> MIRAVFFDSPGTLNSVEGHAKMHLKIMEEVLGDYPLNPKTLLDEYNKLTREAFSNYAGKPYRGLRDILEEVMRKLAEKYGFKYPENFWEISLRMSQRYGELYPEVVEVLKSLKGKYHVGMITDSGTEQAM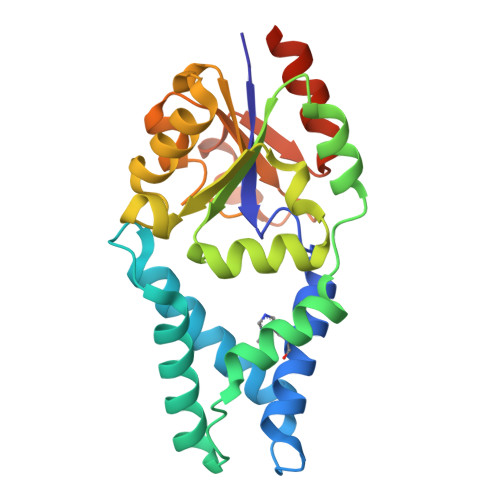AFLDALGIKDLFDSITTSEEAGFFKPHPRIFELALKKAGVKGEEAVYVGDNPVKDAGGSKNLGMTSILLDRKGEKREFWDKADFIVSDLREVIKIVDELNGQGSLEHHHHHH> AAGVEYPANRLANISELTLNEPLDVAYPDEDAAGVLLKLGTRVEGGVGPDGDIVGFSTICPHKGAPLSYSADNKTFNCPGHFSVFDPEKGGQQVWGQATQNLPQYVLRVADNGDIFAEGVDELIYGRLSNV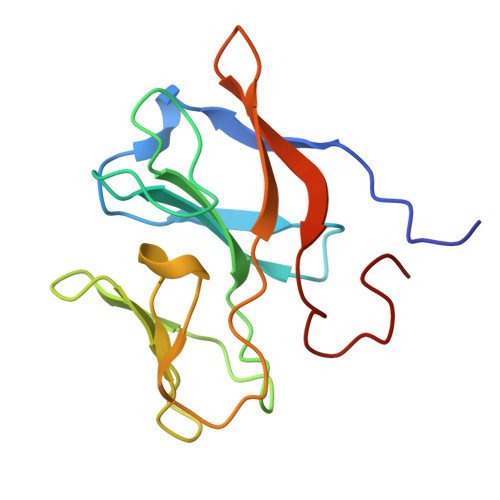L> GPHMRQDIPIEARMNEIVHSLKSRGTRINFM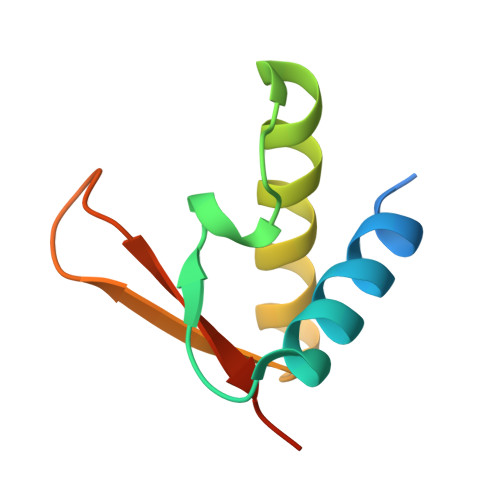DLFPYEQKEHLVVTFLAVLELMKNQLVLIEQEHNFSDIYITGSESIHGA>[2x]KIKACIDEVTTTLEETKFLTNKLLLFADINGKLYHDSQNMLRGEDMSFLEKDAPYMVGDVITSGDITCVVIPSKKAGGTTEMLSRALKKVPVDEYITTYPGQGCAGYTLEEAKTALKKCKSAFYVLPSEAPNAKEEILGTVSWNLREMLAHAEETRKLMPICMDVRAIMATIQRKYKGIKIQEGIVDYGVRFFFYTSKEPVASIITKLNSLNEPLVTMPIGYVTHGFNLEEA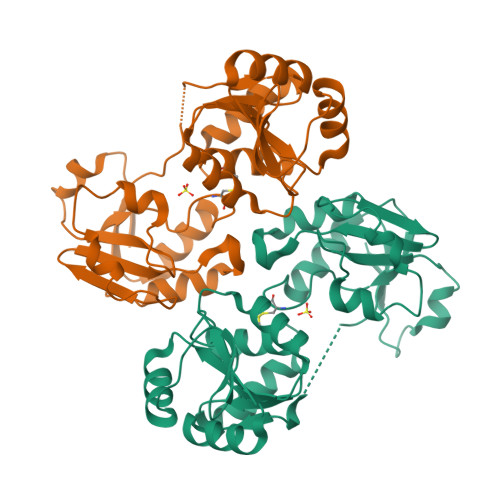ARCMRSLRAPAVVSVSSPDAVTTYNGYLTSSS~{N}-[(1-fluoranylcyclohexyl)methyl]-~{N}-methyl-4-(2-methylsulfanylphenyl)-2-methylsulfonyl-benzamide 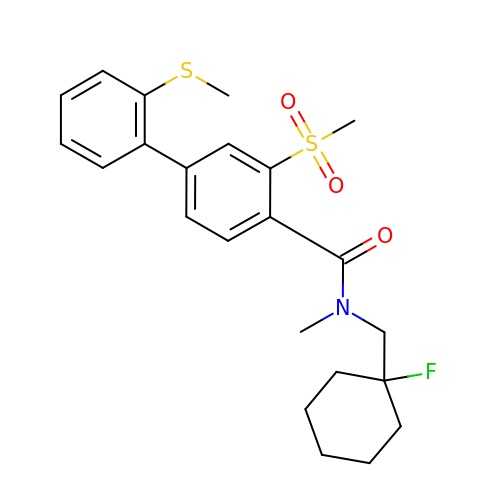| C23 H28 F N O3 S2 | PAFGSEZHUCSUMW-UHFFFAOYSA-N>[2x]GHMSLSKKRKLESGDSGGAGAGGEGAEEENGGEQEAAPPRPRRTKSERDQLYYECYSDVSVHEEMIADQVRTEAYRLGILKNWAALRGKTVLDVGAGTGILSIFCAQAGARRVYAVEASAIWQQAREVVRLNGLEDRVHVLPGPVETVELPERVDAIVSEWMGYGLLHESMLSSVLHARTKWLKE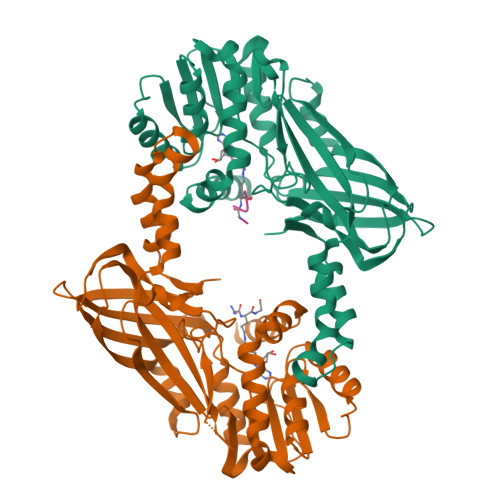GGLLLPASAELFVAPISDQMLEWRLGFWSQVKQHYGVDMSCMESFATRCLMGHSEIVVQDLSGEDVLARPQRFAQLELARAGLEQELEAGVGGRFRCSCYGSAPLHGFAVWFQVTFPGGDSEKPLVLSTSPLHPATHWKQALLYLNEPVPVEQDTDISGEITLLPSPDNPRRLRILLRYKVGDHEEKTKDFAMED;>SGXGKGG[2x]RIBAVIRIN MONOPHOSPHATE 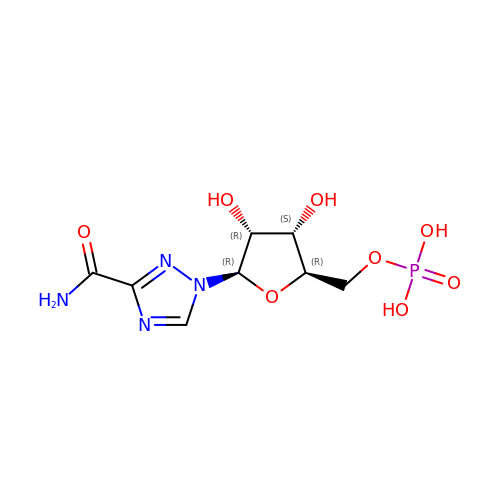| C8 H13 N4 O8 P | SDWIOXKHTFOULX-AFCXAGJDSA-N> SEISRQEFQRRRQALVEQMQPGSAALIFAAPEVTRSADSEYPYRQNSDFWYFTGFNEPEAVLVLIKSDDTHNHSVLFNRVRDLTAEIWFGRRLGQDAAPEKLGVDRALAFSEINQQLYQLLNGLDVVYHAQGEYAYADVIVNSALEKLRKGSRQNLTAPATMIDWRPVVHEMRLFKSPEEIAVLRRAGEITAMAHTRAMEKCRPGMFEYHLEGEIHHEFNRHGARYPSYNTIVGSGENGCILHYTENECEMRDGDLVLIDAGCEYKGYAGAITRTFPVNGKFTQAQREIYDIVLESLETSLRLYRPGTSILEVTGEVVRIMVSGLVKLGILKGDVDELIAQNAHRPFFMHGLSHWLGLDVHDVGVYGQDRSRILEPGMVLTVEPGLYIAPDAEVPEQYRGIG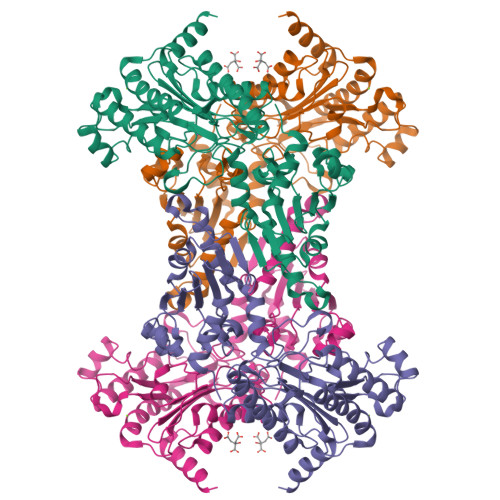IRIEDDIVITETGNENLTASVVKKPEEIEALMVAARKQ>[2x]SNAMTKSRFFSDVAETSSFVFAVAGADDEVVLETIRLALKQKLGKFLLFGKKEDKTLTANESVTWIQTDTAEAAAQGAILAVKNKEADILVKGFIPTATLMHHVLKKENGLRTDQLLSQIAIFDIPTYHKPLLITDCAMNVAPKTKEKIAITENALAVAHQIGITNPKIALLSAVEEVTAKMPSTLEAQEVVQHFGNQISVSGPLALDVAISKEAALHKGITDSSAGEADILIAP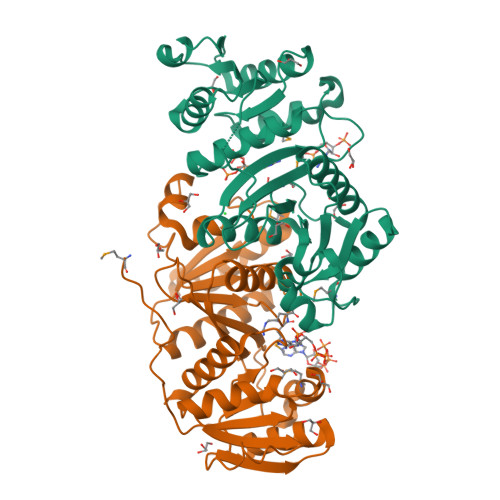NIETGNALYKSLVYFAGAKVGSAVVGAKVPIVISSRNDSPENKLASFILTVRLVEK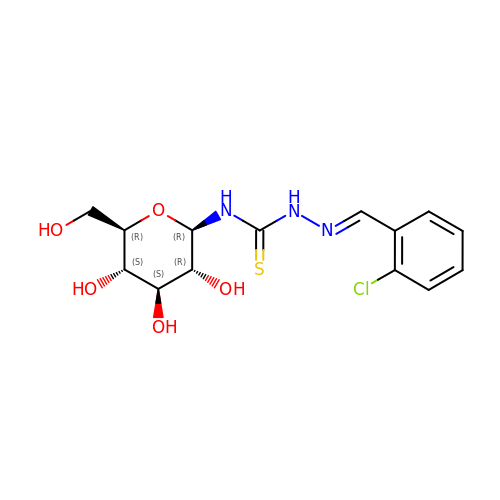N-({(2E)-2-[(2-chlorophenyl)methylidene]hydrazino}carbonothioyl)-beta-D-glucopyranosylamine | C14 H18 Cl N3 O5 S | HKDGHOCNKASZRS-QCOQDYPWSA-N3-(2-aminophenyl)-3-oxopropanoic 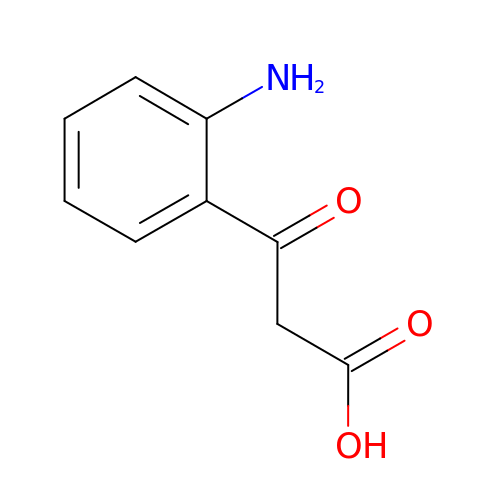acid | C9 H9 N O3 | POAXUNDIOGWQOC-UHFFFAOYSA-N>[2x]TAHRFLFV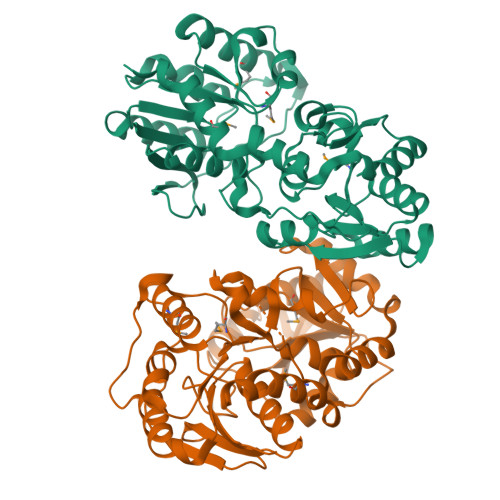STPVGPLGSGRGGGVELTLPNLAKALTQRGHQVSVLAPAGSVLPDLPLETVPGTWQSTAQSHGRATPAEIPAESVLARLWDRAHQQQADFDLILNFAYDWLPLYLTPFFKTPVAHLISMGSLSEVMDQAIATSLDRYPGSIAVHSLAQAATFPFGDRCLCIGNALDLAAYGFNPEPEPVLGWVGRIAPEKGLEDAIQAAQQAGLPLRVWGALTEPDYWQRLQQQFGDRAVSYQGFVSTDELQRGLGRCQGLLMTPKWVEAFGNVAIEALACGLPVIAYARGGPLEIIEQGKSGWLVEPDQQAALVNAIGQLSSLDRAYCRAQAEARFSLAAMGQRLEAWLLPLLS4-({4-[(2,4,6-trimethylphenyl)amino]-1,3,5-triazin-2-yl}amino)benzonitrile 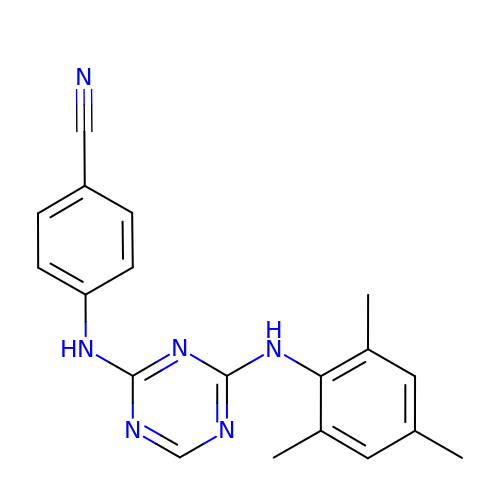| C19 H18 N6 | SOPKWXMQSHLEKD-UHFFFAOYSA-N>[3x]MRLYSNRDRPNHLGPLAL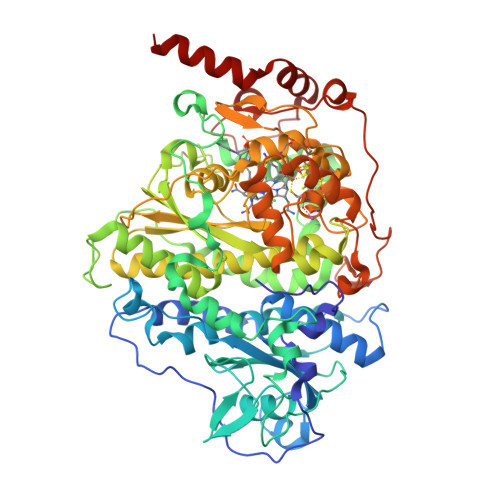ERLARVDDVVAQPARQPEDGFAASEDSLLGDVEEYARLFTRFLDGPVAPLGDAIPDDPARRAENLKASAYFLDASMVGICRLDPDDRAGDCDPSHTHALVFAVQFGREPEAGEAGAEWIRGTNAARTDMRCAEIAAILSGYVRWMGFPARGHFSGDAQVDLARLAVRAGLARVVDGVLVAPFLRRGFRLGVVTTGYALAADRPLAPEGDLGETAPEVMLGIDGTRPGWEDAEEEKRPLHMGRYPMETIRRVDEPTTLVVRQEIQRVAKRGDFFKRAEAGDLGEKAKQEKKRFPMKHPLALGMQPLIQNMVPLQGTREKLAPTGKGGDLSDPGRNAEAIKALGYYLGADFVGICRAEPWMYYASDEVEGKPIEAYHDYAVVMLIDQGYETMEGASGDDWISASQSMRAYMRGAEIAGVMAAHCRRMGYSARSHSNAHSEVIHNPAILMAGLGEVSRIGDTLLNPFIGPRSKSIVFTTDLPMSVDRPIDFGLQDFCNQCRKCARECPCNAISFGDKVMFNGYEIWKADVEKCTKYRVTQMKGSACGRCMKMCPWNREDTVEGRRLAELSIKVPEARAAIIAMDDALQNGKRNLIKRWWFDLEVIDGVAGAPRMGTNERDLSPDRGDKIGANQKLAMYPPRLQPPPGTTLDAVLPVDRSGGLAEYAAAETPAAARARLKSSAGHHHHHH> SNISRQAYADMFGPTVGDKVRLADTELWIEVEDDLTTYGEEVKFGGGKVIRDGMGQGQMLAADCVDLVLTNALIVDHWGIVKADIGVKDGRIFAIGKAGNPDIQPNVTIPIGAATEVIAAEGKIVTAGGIDTHIHWICPQQAEEALVSGVTTMVGGGTGPAAGTHATTCTPGPWYISRMLQAADSLPVNIGLLGKGNVSQPDALREQVAAGVIGLKIH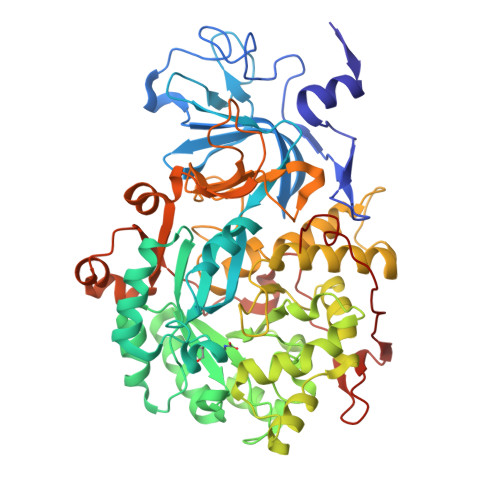EDWGATPAAIDCALTVADEMDIQVALHSDTLNESGFVEDTLAAIGGRTIHTFHTEGAGGGHAPDIITACAHPNILPSSTNPTLPYTLNTIDEHLDMLMVCHHLDPDIAEDVAFAESRIRRETIAAEDVLHDLGAFSLTSSDSQAMGRVGEVILRTWQVAHRMKVQRGALAEETGDNDNFRVKRYIAKYTINPALTHGIAHEVGSIEVGKLADLVVWSPAFFGVKPATVIKGGMIAIAPMGDINASIPTPQPVHYRPMFGALGSARHHCRLTFLSQAAAANGVAERLNLRSAIAVVKGCRTVQKADMVHNSLQPNITVDAQTYEVRVDGELITSEPADVLPMAQRYFLF> SMQRTVARDITLLECVGKGRYGEVWRGSWQGENVAVKIFSSRDEKSWFRETELYN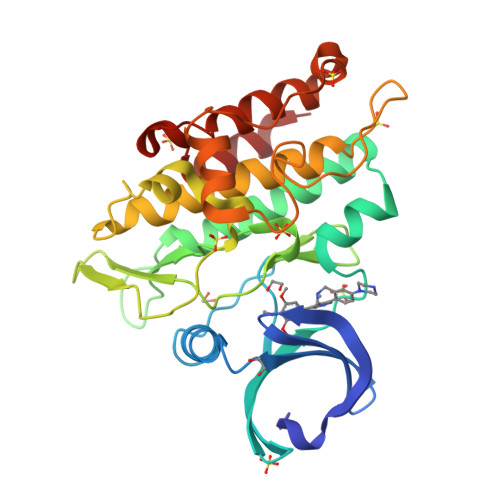TVMLRHENILGFIASDMTSRHSSTQLWLITHYHEMGSLYDYLQLTTLDTVSCLRIVLSIASGLAHLHIEIFGTQGKPAIAHRDLKSKNILVKKNGQCCIADLGLAVMHSQSTNQLDVGNNPRVGTKRYMAPEVLDETIQVDCFDSYKRVDIWAFGLVLWEVARRMVSNGIVEDYKPPFYDVVPNDPSFEDMRKVVCVDQQRPNIPNRWFSDPTLTSLAKLMKECWYQNPSARLTALRIKKTLTKID>KHSLPDLPYDYGALEPHINAQIMQLHHSKNHAAYVNNLNVTEEKYQEALAKGDVTAQIALQPALKFNGGGHINHSIFWTNLSPNGGGEPKGELLEAIKRDFGSFDKFKEKLTAASVGVQGSGWGWLGFNKERGHLQIAACPNQDPLQGTTGLIPLLGIDVWEHAYYLQYKNVRPDYLKAIWNVINWENVTERY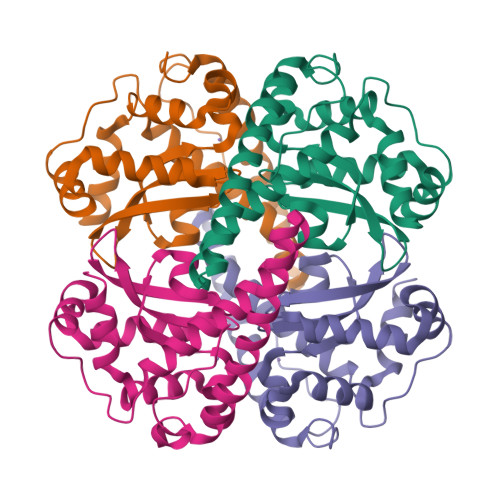MACKK[4x]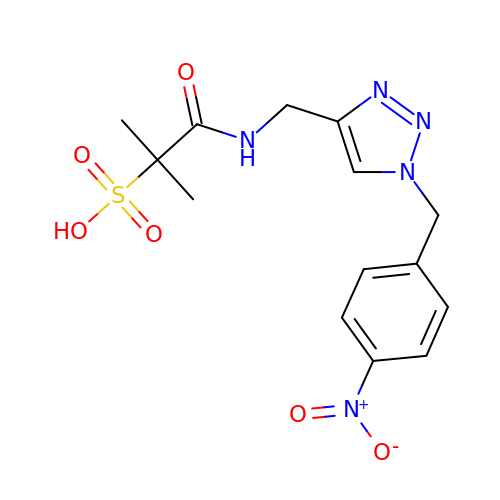2-methyl-1-[[1-[(4-nitrophenyl)methyl]-1,2,3-triazol-4-yl]methylamino]-1-oxidanylidene-propane-2-sulfonic acid | C14 H17 N5 O6 S | SEUUEKSOVBZGDT-UHFFFAOYSA-N> DQ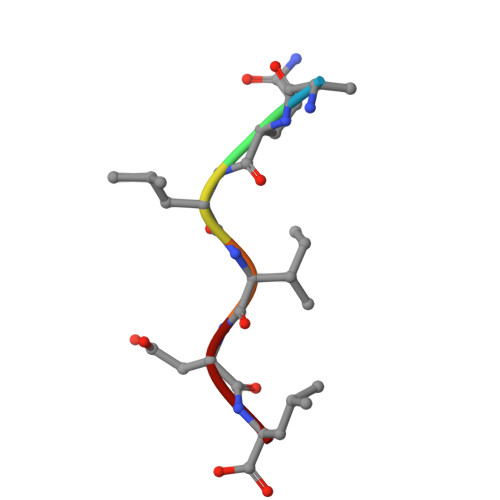LIDL β-Lactam-containing compounds remain the most important antibiotics in clinical use, but their effectiveness is threatened by increasing resistance. β-Lactam resistance is most importantly mediated by serine- and zinc-dependent metallo-β-lactamases (SBLs and MBLs, respectively), which catalyze β-lactam hydrolysis. B1 MBLs (e.g., imipenemase [IMP], Verona integron-encoded MBL [VIM], and New Delhi MBL [NDM] types) are the most clinically relevant MBLs; these MBLs catalyze hydrolysis of almost all β-lactams, including the latest generations of cephalosporins and carbapenems. Crystal structures reveal that MBLs have a characteristic αβ/βα sandwich fold, that they possess conserved zinc ion binding sites, and that loops flanking the active site are involved in ligand binding. We report systematic studies on the inhibition of four clinically relevant MBLs (IMP-1, VIM-2, SPM-1, and NDM-1) and the model MBL BcII by the four captopril stereoisomers and both enantiomers of a captopril derivative, 1-(2-mercaptobenzoyl)pyrrolidine-2-carboxylic acid (d- and l-MBP).

For comparison, structures of di-Zn(II)–VIM-2 and di-Zn(II)–BcII without inhibitors were also determined, to 1.20- and 1.30-Å resolutions, respectively. The active sites, which are located at one end of the two β-sheets in a groove surrounded by several loops, were occupied in all cases by two zinc ions, as expected for B1 subclass MBLs. An interzinc distance of 3.5 Å was observed for both our di-Zn(II)–BcII and di-Zn(II)–VIM-2 apo structures, in which a bridging water was present as previously observed. Preliminary structural analysis indicated that partial oxidation of the metal-binding cysteine (Cys221) had occurred in both the crystallized BcII and VIM-2 proteins, in a manner similar to that observed in previous crystallographic studies of these B1 MBLs. Due to the likelihood of active site cysteine oxidation (Cys221) interfering with the active site Zn(II) chemistry, and hence with our analysis of ligand binding, we worked to minimize Cys221 oxidation. In all cases, cysteine oxidation during crystallization could be prevented by the addition of tris(2-carboxyethyl)phosphine (TCEP) (except for IMP-1, for which cysteine oxidation in the absence of TCEP was not observed). Comparison of the MBL-captopril complex structures with the active site of apo-MBLs reveals that several water molecules are displaced upon binding of d- or l-captopril; these displacements likely contribute to the strength of inhibitor binding.

> SQKVEKTVIKNETGTISISQLNKNVWVHTELGSFDGEAVPSNGLVLNTSKGLVLVDSSWDDKLTKELIEMVEKKFQKRVTDVIITHAHADRIGGIKTLKERGIKAHSTALTAELAKKNGYEEPLGDLQTVTNLKFGNMKVETFYPGKGHTEDNIVVWLPQYNILVGGCLVKSTSAKDLGNVADAYVNEWSTSIENVLKRYRNINAVVPGHGEVGDKGLLLHTLDLLK>[2x]SCSKCRKEMGQVEISSCTVDRDTVCGCRKNQYRHYWSENLFQCFN

Here, we describe the chemical synthesis and folding of a central, cysteine-rich domain of the cell-surface receptor tumor necrosis factor 1 which is integral to binding of the cytokine TNF-α, namely, TNFR-1 CRD2. As this central portion of the receptor contains a significant number of TNF-α interface residues,11b we envisioned that it can be synthesized individually and serve as a truncated mimic for the TNFR-1. Cell-surface receptors, responsible for converting external stimuli to cellular responses, are critical targets for physiological investigations as well as diagnostics and therapeutics design. While recombinant routes for preparing receptors are most frequently used, chemical protein synthesis has unique advantages for research by offering atomistic control and fully breaking the barrier of chirality.

Here, we present a synthetic route to the TNFR-1 CRD2 protein domain using a one-pot chemical ligation and refolding procedure. As the linear TNFR-1 CRD2 polypeptide contains six cysteine residues, there are 15 possible combinations for disulfide bond formation. The highest refolding yield (33% by HPLC) was achieved by preparing a solution of TNFR-1 CRD2 (0.5 mg/mL) in 6 M Gdn·HCl, 0.1 M sodium phosphate buffer (pH 6.5), 6 mM glutathione disulfide, and 60 mM glutathione, which was then rapidly diluted 5-fold with 0.1 M phosphate buffer (pH 6.5). Subsequently, we conducted racemic protein crystallography to analyze the structure of TNFR-1 CRD2.4 This technique involves crystallizing small proteins from a racemic protein mixture to gain prompt access of high-resolution structural data.15d,17 Here, enantiomeric TNFR-1 CRD2, prepared entirely from d-amino acids (d-TNFR-1 CRD2), was synthesized following the protocol developed above with an overall yield of 16%. The racemic TNFR-1 CRD2 mixture was subjected to sparse matrix crystallization screening, and the best crystal-forming condition was identified to contain 25 mg/mL of protein racemate, 1.5 M sodium chloride, and 10% v/v ethanol. The crystal structure was solved at 1.4 Å resolution, confirming the correct disulfide bond patterns with well-defined electron density. The TNFR-1 CRD2 structure aligned well with that of the entire receptor TNFR-1 in complex with TNF-α,11c showing a backbone root-mean-square deviation (RMSD) of 0.36 Å across the cytokine binding interface. The binding experiments with human TNF-α (Peprotech) showed clear binding to l-TNFR-1 CRD2 (KD ≈ 7 nM), with no binding to the d-counterpart. Consequently, this indicated that the TNFR-1 CRD2 is structurally conserved, and its binding to TNF-α suggested that it can serve as a receptor mimic for further investigations.3-(3-cyclohexyl-3,8,10-triazatricyclo[7.3.0.0^{2,6}]dodeca-1,4,6,8,11-pentaen-5-yl)benzenesulfonyl 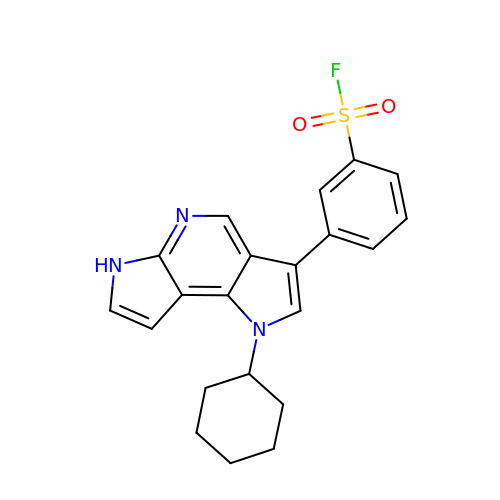fluoride | C21 H20 F N3 O2 S | HVHFAYSIIPDURH-UHFFFAOYSA-N>[2x]EFPEITEEMEKEIKNVFRNGNQDEVLSEAFRLTITRKDIQTLNHLNWLNDEIINFYMNMLMERSKEKGLPSVHAFNTFFFTKLKTAGYQAVK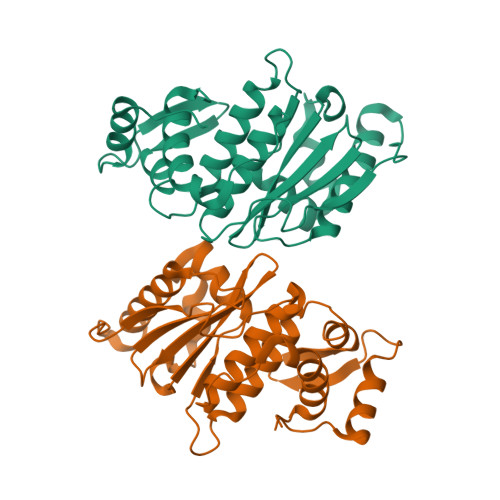RWTKKVDVFSVDILLVPIHLGVHWCLAVVDFRKKNITYYDSMGGINNEACRILLQYLKQESIDKKRKEFDTNGWQLFSKKSQEIPQQMNGSDCGMFACKYADCITKDRPINFTQQHMPYFRKRMVWEILHRKLL> MTAKDDYPSLSFQQDYVYIFSSDFQLSEELGVALINA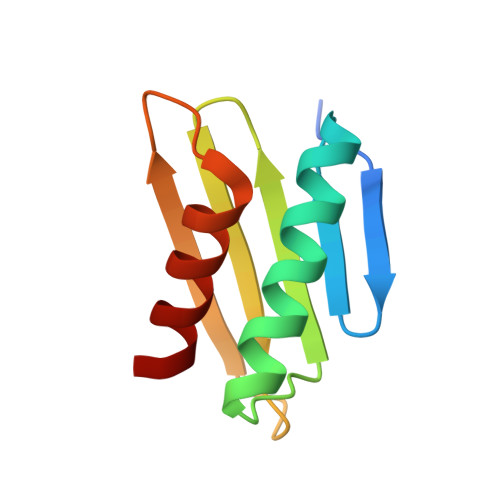LSAKEIVPERLYVMLNDKTISFSFISKNKKSKNRVLSTEKKLNYKHISEYIVNEIEY6-amino-2H-chromen-2-one | C9 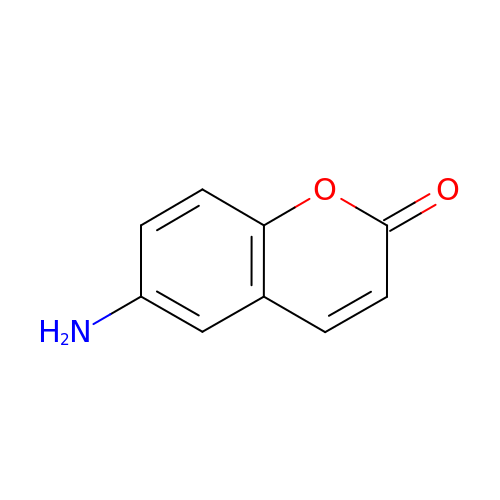H7 N O2 | ZOJAINJCZSVZGW-UHFFFAOYSA-N2-(trifluoromethyl)-1H-benzimidazol-7-ol | C8 H5 F3 N2 O | 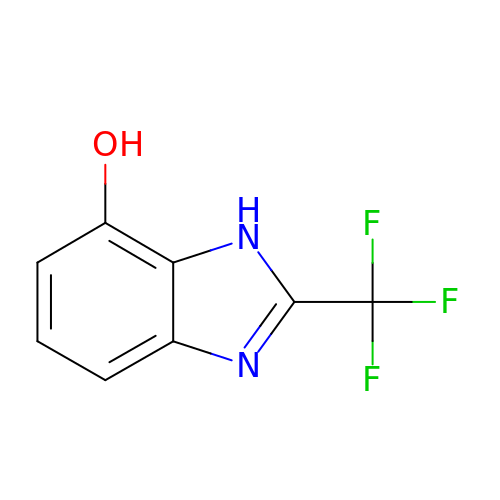LHFTYTVRWFFRAR-UHFFFAOYSA-N>[2x]PPLDLNNIQGD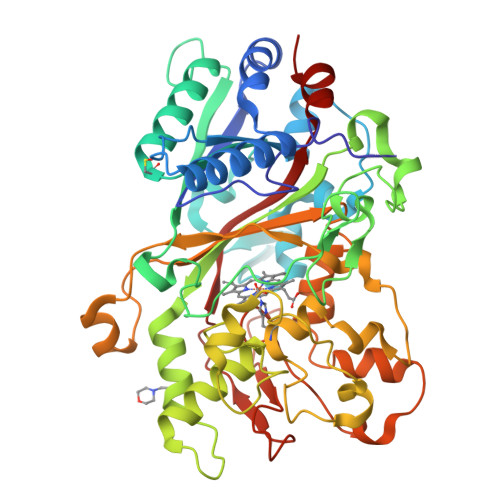ILGGLPKRTETYFFFDVTNVDQFKANMAHFIPHIKTSAGIIKDREAIKEHKRQKKPGLVPMAAVNVSFSHLGLQKLGITDDLSDNAFTTGQRKDAEILGDPGSKNGDAFTPAWEAPFLKDIHGVIFVAGDCHGSVNKKLDEIKHIFGVGTSHASISEVTHVRGDVRPGDVHAHEHFGYLDGISHPAVEQFDQNPLPGQDPIRPGFILAKENGDSRAAARPDWAKDGSFLTFRYLFQMVPEFDDFLESNPIVLPGLSRKEGSELLGARIVGRWKSGAPIEITPLKDDPKLAADAQRNNKFDFGDSLVRGDQTKCPFAAHIRKTYPRNDLEGPPLKADIDNRRIIRRGIQFGPEVTSQEHHDKKTHHGRGLLFVCYSSSIDDGFHFIQESWANAPNFPVNAVTSAGPIPPLDGVVPGFDAIIGQKVGGGIRQISGTNPNDPTTNITLPDQDFVVPRGGEYFFSPSITALKTKFAI> GSSPVQSGFNNGTISNYMYFERRPDLLTKGTQDKAAAVKLKIENFYQSSVKYAIERNERRVELETELTSHNWSEERKSRQLSSLGKKESQFLRLRRTRLSLEDFHTVKVIGKGAFGEVRLVQKKDTGKIYAMKTLLKSEMYKKDQLAHVKAERDVLAGSDSPWVVSLYYSFQDAQYLYLIMEFLPGGDLMTMLIRWQLFTEDVTRFYMAECILAIETIHKLGFIHRAIKPDNILIDIRGHIKLSDFGLSTGFHKTHDSNYYKKLLQQDEATNGISKPGTYNANTTDTANKRQTMVVDSISLTMSNRQQIQTWRKSRRLMAYSTVGTPDYIAPEIFLYQGYGQECDWWSLGAIMYECLIGWPPFCSETPQETYRKIMNFEQTLQFPDDIHISYEAEDLI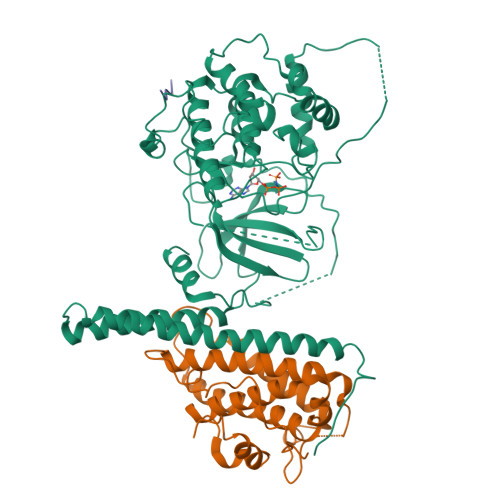RRLLTHADQRLGRHGGADEIKSHPFFRGVDWNTIRQVEAPYIPKLSSITDTRFFPTDELENVPDSPAMAQAAKQREQMTKQGGSAPVKEDLPFIGYTYSRFDYLTRKNAL;> GSRNKHHSPKRHSQTSFPAQKSTPQSQQLTSTTPQSQQQEASERSESQQIMFLSEPFVRTALVKGSFKTIVQLPKYVDLGEWIALNVFEFFTNLNQFYGVVAEYVTPDAYPTMNAGPHTDYLWLDANNRQVSLPASQYIDLALTWINNKVNDKNLFPTKNGLPFPQQFSRDVQRIMVQMFRIFAHIYHHHFDKIVHLSLEAHWNSFFSHFISFAKEFKIIDRKEMAPLLPLIESFEKQGKIIYN;> TTEQSDFKFP> MAINFKGSPYLDRFDPSKDRTKVLFNPDRPLQQAELNEMQSIDQYYLKNLGDAIFKDGDKQSGLGFTLSEDNVLTVNPGYVYINGKIRYYDNDDSVKITGVGKETIGIKLTERIVTPDEDASLLDQTSGVPSYFSKGADRLEEKMSLTVNDPTSATIYTFMDGDLYIQSTNAEMDKINKVLAERTYDESGSYKVNGFELFSEGNAEDDDHVSVVVDAGKAYVKGFKVDKPVSTRISVPKSYDLGTAENESTIFNKSNNSISLANSPVKEIRRVTGQVLIEKERVTRGAQGDGQDFLSNNTAFEIVKVWTETSPGVTTKEYKQGEDFRLTDGQTIDWSPQGQEPSGGTSYYVSYKYNKRMEAGKDYEVTTQGEGLSKKWYINFTPSNGAKPIDQTVVLVDYTYYLARKDSVFINKYGDIAILPGEPNIMRLVTPPLNTDPENLQLGTVTVLPDSDEAVCISFAITRLS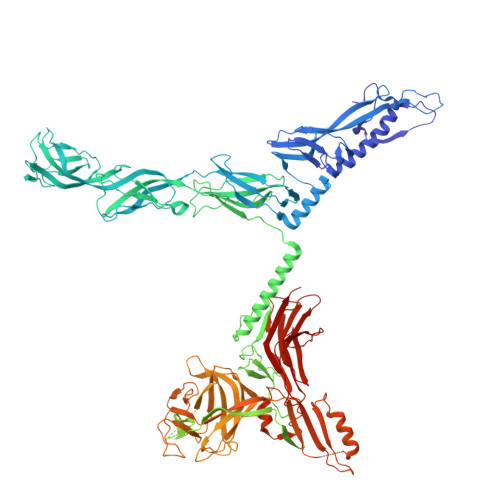MEDLQKVKTRVDNLEYNQAVNALDDGAMEGQNPLTLRSVFSEGFISLDKADITHPDFGIVFSFEDAEATLAYTEAVNQPKIIPGDTTAHIWGRLISAPFTEERTIYQGQASETLNVNPYNIPNKQGVLKLTPSEDNWIDTENVTITEQKTKKVTMKRFWRHNESYYGETEHYLYSNLQLDAGQKWKGETYAYDREHGRTGTLLESGGQRTLEEMIEFIRIRDVSFEVKGLNPNDNNLYLLFDGVRCAITPATGYRKGSEDGTIMTDAKGTAKGKFTIPAGIRCGNREVTLKNANSTSATTYTAQGRKKTAQDIIIRTRVTVNLVDPLAQSFQYDENRTISSLGLYFASKGDKQSNVVIQIRGMGDQGYPNKTIYAETVMNADDIKVSNNASAETRVYFDDPMMAEGGKEYAIVIITENSDYTMWVGTRTKPKIDKPNEVISGNPYLQGVLFSSSNASTWTPHQNSDLKFGIYTSKFNETATIEFEPIKDVSADRIVLMSTYLTPERTGCTWEMKLILDDMASSTTFDQLKWEPIGNYQDLDVLGLARQVKLRATFESNRYISPLMSSSDLTFTTFLTELTGSYVGRAIDMTEAPYNTVRFSYEAFLPKGTKVVPKYSADDGKTWKTFTKSPTTTRANNEFTRYVIDEKVKSSGTNTKLQVRLDLSTENSFLRPRVRRLMVTTRDE Here we report the biochemical and structural characterization of this M-ADH enzyme, which we refer to as BkTauF. We demonstrate that it is a novel sulfoacetaldehyde reductase, which differs from BwSarD in active site residues and metabolic function. BkTauF catalyzed both sulfoacetaldehyde reduction and isethionate oxidation, as measured using a continuous spectrophotometric assay monitoring the decrease/increase in absorbance at 340 nm due to consumption/production of NAD(P)H. The optimal reaction pH for sulfoacetaldehyde reduction was 7.5, while that for isethionate oxidation was 10.0. Each monomer consists of an N-terminal domain (α1–α5 and β1–β9; residues 1–178) with Rossmann fold, and a C-terminal helical domain (α6-α14; residues 179–375), similar to other structurally characterized M-ADH enzymes.

Crystal structures of BkTauF, both in the apo form and in complex with the NAD+ cofactor, were solved at 1.9 and 3.0 Å resolution, respectively. The apo and NAD+-bound structures are nearly identical, with RMSD of 0.37 Å over 375 Cα atoms. The asymmetric unit contains four monomers. The quaternary prediction server PISA suggests that BkTauF forms a dimer, consistent with its oligomeric state in solution determined by gel filtration chromatography. Out of the four monomers in the asymmetric unit, only one contains the catalytic Zn(II) ion, coordinated to Asp192, Gln196, His261 and His275. Catalytic activity of BkTauF was abolished by chelation with EDTA, and recovered up to 85% by addition of Zn2+ and 15% by addition of Fe2+, suggesting that the physiological metal cofactor for BkTauF is Zn2+. Furthermore, the putative isethionate-binding site adjacent to the catalytic Zn2+ is very open, which precluded molecular docking. The present crystal structure could represent an ‘open’ conformation, and further conformational changes could occur subsequent to isethionate binding to form an enclosed active site resembling that of other M-ADH enzymes like FucO.

>[4x]SNGGGMLWDYAQPVTIRFGKGRAMEIKDIAEAMGLHDGIMVTPKFFVDSGEAQRLIDASDGAVSTVFTDFSPNPDVTEVDACAEIIRKNHCEFVVAMGGGSAMDVSKAAASICLTDDSIADYHGTGKAMPQKHLPIIALPTTAGTGSEVTCVSVLTNRKLGKKAPIVSDGFFPSVAIVDPELTYSVPPKITASTGMDVLSQAIEGFWSKGHQPICDSCAAHAAKLVFKYLPIAVAEPHNEEAREKMCEASVIAGLAFTLPKTTSSHACSFPLTNIHGIPHGEACGLTLDYFARINKDAQHGRVQEFARGIGFKDVDAMADAIHDLKVRIGMRTGLKDLNLTEEQIADLVRISRHPNLYNNPVEITDDMLDTMYHYLASTD N-oleoyl-D-erythro-sphingosylphosphorylcholine | C41 H82 N2 O6 P | 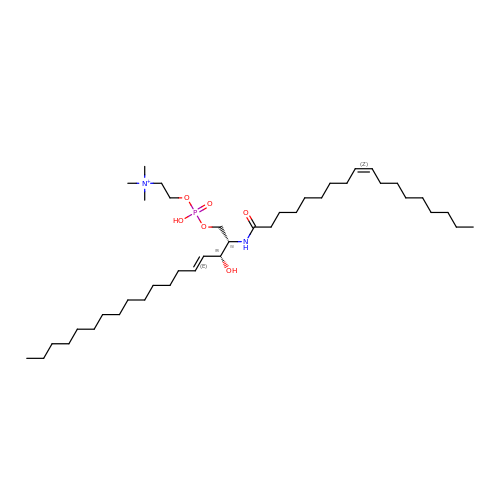NBEADXWAAWCCDG-QDDWGVBQSA-O> MMETERLVLPPPDPLDLPLRAVELGCTGHWELLNLPGAPESSLPHGLPPCAPDLQQEAEQLFLSSPAWLPLHGVEHSARKWQRKTDPWSLLAVLGAPVPSDLQAQRHPTTGQILGYKEVLLENTNLSATTSLSLRRPPGPASQSLWGNPTQYPFWPGGMDEPTITDLNTREEAEEEIDFEKDLLTIPPGFKKGMDFAPKDCPTPAPGLLSLSCMLEPLDLGGGDEDENEAVGQPGGPRGDTVSASPCSAPLARASSLEDLVLKEASTAVSTPEAPEPPSQEQWAIPVDATSPVGDFYRLIPQPAFQWAFEPDVFQKQAILHLERHDSVFVAAHTSAGKTVVAEYAIALAQKHMTRTIYTSPIKALSNQKFRDFRNTFGDVGLLTGDVQLHPEASCLIMTTEILRSMLYSGSDVIRDLEWVIFDEVHYINDVERGVVWEEVLIMLPDHVSIILLSATVPNALEFADWIGRLKRRQIYVISTVTRPVPLEHYLFTGNSSKTQGELFLLLDSRGAFHTKGYYAAVEAKKERMSKHAQTFGAKQPTHQGGPAQDRGVYLSLLASLRTRAQLPVVVFTFSRGRCDEQASGLTSLDLTTSSEKSEIHLFLQRCLARLRGSDRQLP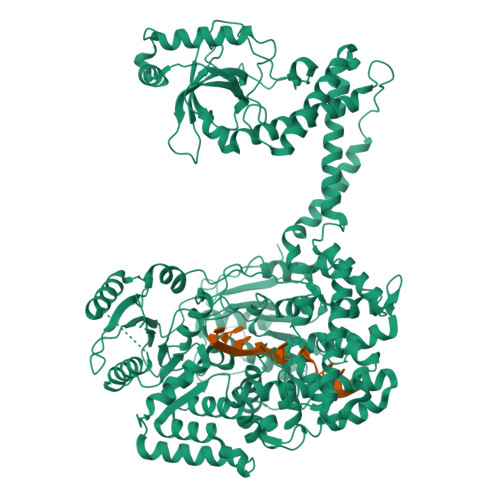QVLHMSELLNRGLGVHHSGILPILKEIVEMLFSRGLVKVLFATETFAMGVNMPARTVVFDSMRKHDGSTFRDLLPGEYVQMAGRAGRRGLDPTGTVILLCKGRVPEMADLHRMMMGKPSQLQSQFRLTYTMILNLLRVDALRVEDMMKRSFSEFPSRKDSKAHEQALAELTKRLGALEEPDMTGQLVDLPEYYSWGEELTETQHMIQRRIMESVNGLKSLSAGRVVVVKNQEHHNALGVILQVSSNSTSRVFTTLVLCDKPLSQDPQDRGPATAEVPYPDDLVGFKLFLPEGPCDHTVVKLQPGDMAAITTKVLRVNGEKILEDFSKRQQPKFKKDPPLAAVTTAVQELLRLAQAHPAGPPTLDPVNDLQLKDMSVVEGGLRARKLEELIQGAQCVHSPRFPAQYLKLRERMQIQKEMERLRFLLSDQSLLLLPEYHQRVEVLRTLGYVDEAGTVKLAGRVACAMSSHELLLTELMFDNALSTLRPEEIAALLSGLVCQSPGDAGDQLPNTLKQGIERVRAVAKRIGEVQVACGLNQTVEEFVGELNFGLVEVVYEWARGMPFSELAGLSGTPEGLVVRCIQRLAEMCRSLRGAARLVGEPVLGAKMETAATLLRRDIVFAASLYTQ>[4x]MLK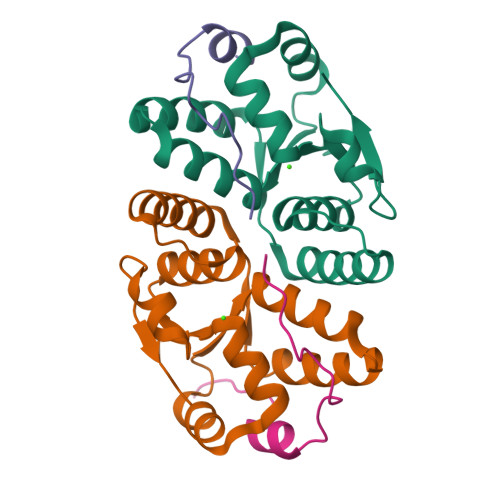FMLDTNTCIFTIKNKPEHIRERFNLNTSRMCISSITLMELIYGAEKSLAPERNLAVVEGFISRLEVLDYDTQAAIHTGQIRAELARKGTPVGPYDQMIAGHAGSRGLVVVTNNLREFERIPGIRIEDWC;>[2x]SWDSWFDGEGASTDFMSTREQP;>[2x]IITPVGESWDSWFDGEGASTDFMSTREQP N-[1-(5-bromo-2,3-dimethoxybenzyl)piperidin-4-yl]-4-sulfanylbutanamide | C18 H27 Br N2 O3 S | 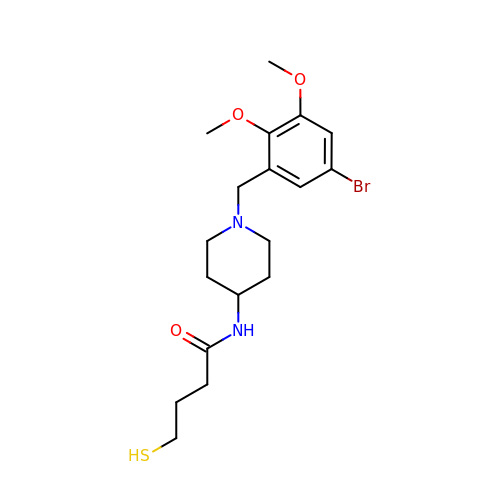HESMISSJMKCCAV-UHFFFAOYSA-N>GHMKGNTMKQLRFGLFENAQTNDSGTATWRHPDNQRHLFDTLDYWRNIAQICEDAGLDFVFLADAWGWADVNGERPDICDVEGLDLPRLDPAIVAAALIASTTKLGLVMTGSTLLEQPYSFARRMASLDHLSKGRIGWNVVTTGTAETASAAFGVPMVAHDDRYDMADDFMELVYKLWEGAWEPDALERDKQGRYADPAKVHRIDHEGPYFRSNGYGNTSYSPQGTPVLFQAGSSERGRQFGGRHGECIFLGGAPIPKLAEQVRAIRAEAVAEGRAADSIKLMAAFSCVIAPTHEEAVQKYQEV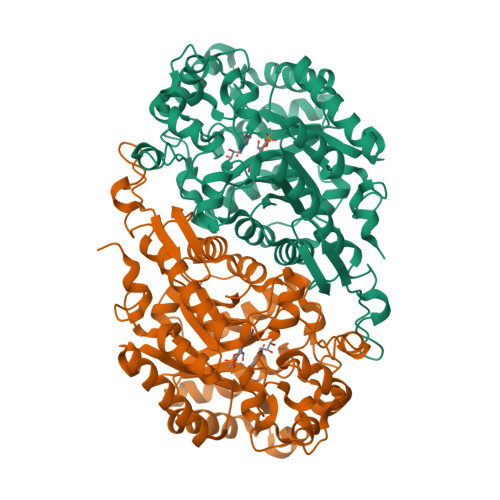LDSQTPEVAVASYAWFTGLDLSSYDPSTPMSELHTELSQTQVARFAGLTVGDVLADWHAHGVRTKPVVGTPEEVADAIVELAEGADLDGFLLTPVIQPGSTIDFIEHVLPILRERGVAASGYDAPTLRERLLGTETPVLREDHPGAGYRAQSGALVG[2x]>[13x]MTNLQDQTQQIVPFIRSLLMPTTGPASIPDDTLEKHTLRSETSTYNLTVGDTGSGLIVFFPGFPG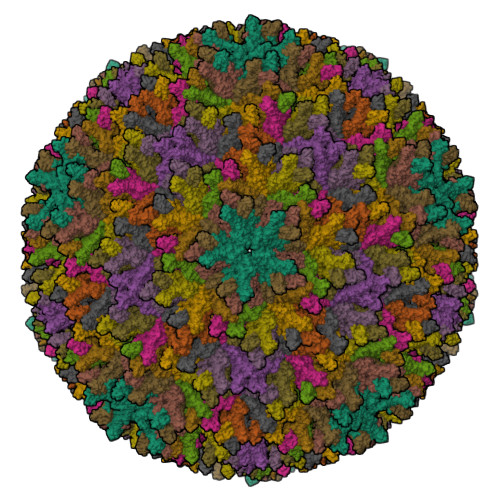SIVGAHYTLQGNGNYKFDQMLLTAQNLPASYNYCRLVSRSLTVRSSTLPGGVYALNGTINAVTFQGSLSELTDVSYNGLMSATANINDKIGNVLVGEGVTVLSLPTSYDLGYVRLGDPIPAIGLDPKMVATCDSSDRPRVYTITAADDYQFSSQYQPGGVTITLFSANIDAITSLSVGGELVFRTSVHGLVLGATIYLIGFDGTTVITRAVAANNGLTTGTDNLMPFNLVIPTNEITQPITSIKLEIVTSKSGGQAGDQMSWSARGSLAVTIHGGNYPGALRPVTLVAYERVATGSVVTVAGVSNFELIPNPELAKNLVTEYGRFDPGAMNYTKLILSERDRLGIKTVWPTREYTDFREYFMEVADLNSPLKIAGA> SNAPPGTVDKKMVEKCWKLMDKVVRLCQNPKLALKNSPPYILDLLPDTYQHLRTILSRYEGKMETLGENEYFRVFMENLMKKTKQTISLFKEGKERMYEENSQPRRNLTKLSLIFSHMLAELKGIFPSGLFQGDTFRITKADAAEFWRKAFGEKTIVPWKSFRQALHEVHPISSGLEAMALKSTIDLTCNDYISVFEFDIFTRLFQPWSSLLRNWNSLA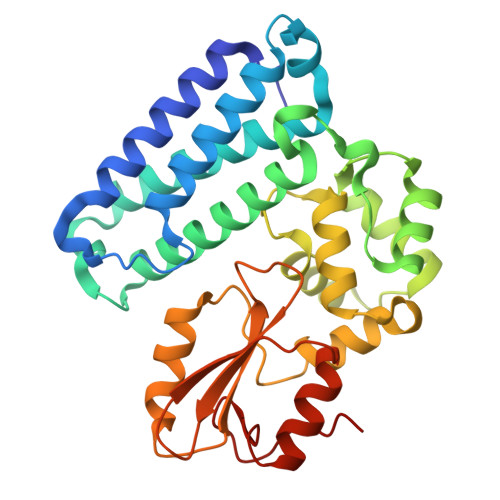VTHPGYMAFLTYDEVKARLQKFIHKPGSYIFRLSCTRLGQWAIGYVTADGNILQTIPHNKPLFQALIDGFREGFYLFPDGRNQNPDLTG> MKLALLASLIASAAAFAPSSSTGAARASTALDAGKKSQALPFLPYPENLAGYVGDAGFDPFRFSDFAPMDFLREAEIKHGRICM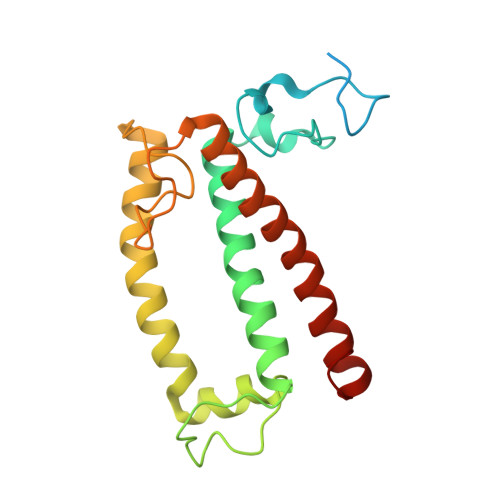LAWLGFVAVDLGARIYPLPEAYEGLTAVTAHDALVQQGAMSQIFLWCSVFEAISTVSVIQMLYEESGREPGYFGFDPLGFLNGKSEAEVNEMKLKEIKNGRLAMLAFSGVVTQAVLTQGPFPYV> MNKDIATPIRTKEI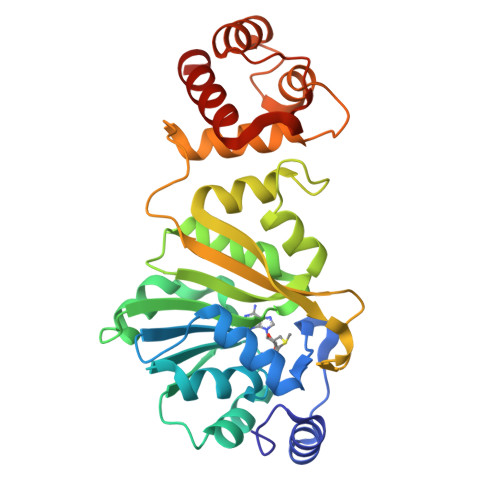LKKYGFSFKKSLGQNFLIDTNILNRIVDHAEVTEKTGVIEIGPGIGALTEQLAKRAKKVVAFEIDQRLLPILKDTLSPYENVTVIHQDVLKADVKSVIEEQFQDCDEIMVVANLPYYVTTPIIMKLLEEHLPLKGIVVMLQKEVAERMAADPSSKEYGSLSIAVQFYTEAKTVMIVPKTVFVPQPNVDSAVIRLILRDGPAVDVENESFFFQLIKASFAQRRKTLLNNLVNNLPEGKAQKSTIEQVLEETNIDGKRRGESLSIEEFAALSNGLYKALF> MRTLFFIPSMGSVRLPLIDFLVKNDIEYVILSRRNHVAVQREIALDMFLEMKDYDTLAFLDEDVVPIEIDFQKVEAKFNEGYDVVCGYYYLKTLRGYSVYRKDWEKEIFDGEVNGCGLGFTFIKREFLEKIKRPAFLAFKPIESPHWIGEDVYFFSTHKPRTYALSSLK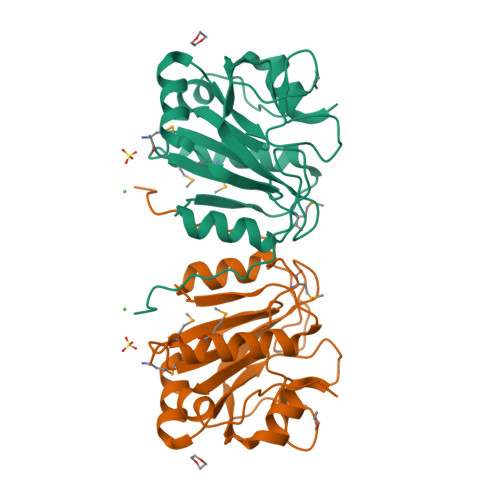AYHFIDERLALSPDRKLILQNDHVARIKHHHHHH>GAGAGAGAGAGMEQTYFISGANRGIGFSVVQRLAAKSGVKVIATARDPASATALNELAKE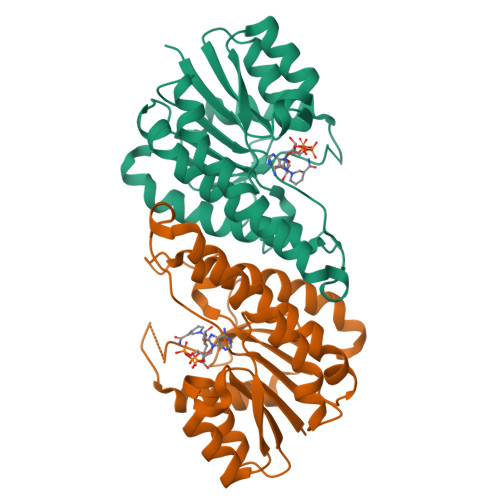NPQVKVVQLDISDEESIKKIAKNVSQYTDSIDVFVSNAAIAKSFGPLLNTPREQWIEHFFTNVLGPIRLFQELYPLIKKGTQKKVFFISSNAGSLNLDFGLDFSAFGQSKAALNYSTKELARQLKPENFIVAAVHPGVVTTDMGKGGERAFTAVDEVSAKKFFTPETKITPEESAAALCKLFESLNTTGKYLSYDGTELPW[4x]The chromophores of reversibly switchable fluorescent proteins (rsFPs) undergo photoisomerization of both the trans and cis forms. Concurrent with cis/trans photoisomerisation, rsFPs typically become protonated on the phenolic oxygen resulting in a blue shift of the absorption. A synthetic rsFP referred to as rsEospa, derived from EosFP family, displays the same spectroscopic behavior as the GFP-like rsFP Dronpa at pH 8.4 and involves the photoconversion between nonfluorescent neutral and fluorescent anionic chromophore states. RsEospa shows cis–trans isomerization at both acidic and neutral pH with similar atomic coordinate modification but distinctively different visible excitation requirements and spectral features.

At pH 5.5 we see a striking difference in the photoswitching behavior. The unilluminated structure shows the cis chromophore, while illumination with 405 nm light accumulates the trans state with high yields. However, at pH 5.5 we observe that the OFF state is identified as the cationic chromophore with additional protonation of the imidazolinone nitrogen which is concurrent with a newly formed hydrogen bond with the Glu212 carboxylate side chain. Excitation of the neutral-cis with 400 nm light causes a bleach in the 389 nm peak and a + 7 nm redshift assigned to the formation of a cationic-trans chromophore. Under the illuminated condition, we observe difference spectra peaks at 1713 and 1692 cm–1 at pH 5.5 and at 1710 and 1690 cm–1 at p2H 5.5 which we assign to the C=O stretch of the cationic-trans chromophore. The DED of the trans structures at pH 8.4 and 5.5 indicate movement of His194 and Glu212 and show significant negative density close to the N4 and C=O of the imidazolinone ring. The Glu212 carboxyl oxygen to imidazolinone-ring nitrogen (N4) distance is reduced from 3.76 Å at pH 8.4 to 2.54 Å at pH 5.5. We interpret this rearrangement as the formation of a H-bond which is made favorable by protonation of the chromophore. We therefore conclude that the majority of trans chromophore structural changes between pH 8.4 and 5.5 are due to the formation a cationic-trans chromophore compared to the neutral. At acidic pH, this isomerization occurs reversibly with a change in protonation state to a trans-cation chromophore state, a new class of reaction not previously observed in rsFPs.

> MSAIKPDMKIKLRMEGNVNGHHFVIDGDGTGKPFEGKQSMDLEVKEGGPLPFAFDILTTAFAYGNRVFAKYPDNIQDYFKQSFPKGYSWERSLTFEDGGICNARNDITMEGDTFYNKVRFYGTNFPANGPVMQKKTLKWEPATEKMYVRDGVLTGDVETALLLEGNAHYRCDFRTTYKAKEKGVKLPGAHFVDHCIEILSHDKDYNKVKLYEHAVAHSGLPDNARR Trypanosoma brucei is the protozoan parasite that is the causative agent of Human African Trypanosomiasis (HAT), also known as African sleeping sickness. However, in T. brucei there are no enzymes for de novo synthesis and this parasite relies solely on its salvage pathways to make its purine nucleoside monophosphates. HGPRT is central to this salvage pathway, as it is responsible for the synthesis of IMP and GMP from hypoxanthine and guanine, respectively. Thus, the crystallographic and SEC-MALLS data agree in demonstrating that TbrHGPRT is dimeric.

In the complex with 6 there are two separate dimers in the asymmetric unit, and in the complex with IMP or 5 two independent subunits are present in the asymmetric unit. The binding of 6 (with five carbons in the linker and hypoxanthine as the base) is similar to that observed for 3 (six carbons in the linker and guanine as the base) in that the purine base binds in the purine binding pocket and the phosphonate moiety binds to the amino acid residues surrounding the 5′-phosphate binding site (residues D117-T121). Compound 6, with hypoxanthine as the base cannot form a hydrogen bond between the exocyclic amino group and the main chain carbonyl of D173. Compared to 3, the purine ring of 6 is translated by ~1 Å, however four hydrogen bonds (two to K145 and two to V167) that hold the purine ring in place are conserved in the two complexes. The phosphonyl oxygen atoms in 6 form hydrogen bonds with the amide nitrogen atoms of D117, T118, A119, L120 and the side-chains of T118 and T121 similar to the binding of one of the conformations of 3. Compound 6 with one fewer carbon atom than 3, is able to reach into the 5′-phosphate binding site with its phosphonate group, thus explaining the similar Ki values for 3 and 6 (15.8 μM vs 21.2 μM). Compound 2 (with guanine as the base) and 6 (with hypoxanthine as the base) both have Ki values significantly lower than their corresponding nucleoside monophosphates, while the remaining five ANPs have Ki values similar to or greater than those for the nucleoside monophosphates. Common to 2 and 6 is the fact that they both have five carbon atoms linking the base to the phosphorus atom and this is a key factor that results in tighter binding compared to the other inhibitors. However, 2 binds more tightly to human HGPRT (0.5 μM vs 2.3 μM), while for 6 the reverse is true since it binds more tightly to TbrHGPRT (>100 μM vs 15.8 μM). For 6 the well solution was 25% PEG 3350, 0.2 M sodium iodide, 0.1 M Bis-Tris propane, pH 6.5.

>HHHHHHMEPACKYDFATSVLFTEAELHTRMRGVAQRIADDYSNCNLKPLENPLVIVSVLKGSFVFTADMVRILGDFGVPTRVEFLRASSYGHDTKSCGRVDVKADGLCDIRGKHVLVLEDILDTALTLREVVDSLKKSEPASIKTLVAIDKPGGRKIPFTAEYVVADVPNVFVVGYGLDYDQSYREVRDVVILKPSVYETWGKELERRKAAGEAKR[4x]> MKTEWPELVGKSVEEAKKVILQDKPAAQIIVLPVGTIVTMEYRIDRV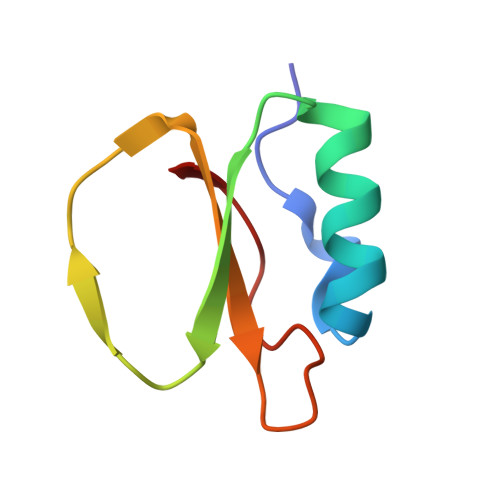ALFVDRLDNIAQVPRVG>[3x]MSELDFLLKKKRKSEDEEKIINNNENAKKEEITNEEEKIKNDMLKYIEKDPKIG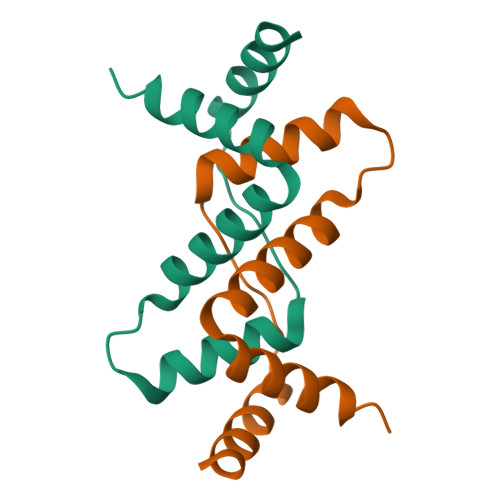VWSYPAFLVLQYLYHTVPGFKMSRTAKEALEKGLKEMYPTLFTIAEKIAKERFKEHHHHHH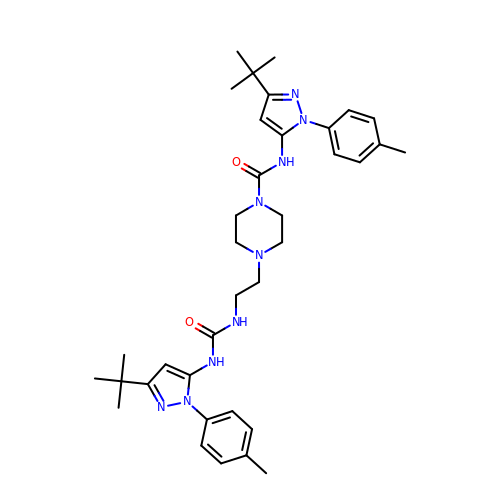N-[3-tert-butyl-1-(4-methylphenyl)-1H-pyrazol-5-yl]-4-[2-({[3-tert-butyl-1-(4-methylphenyl)-1H-pyrazol-5-yl]carbamoyl}amino)ethyl]piperazine-1-carboxamide | C36 H49 N9 O2 | DWTWTHMDBSOYDZ-UHFFFAOYSA-N>GSPSRKFYWRAKSQMCEVKGWVPTHRGFPWGPELPGDLILSRRAYVSCDLTSCFKFFIAYGLSANQHLLNTSMEWEESLYKTPIGSASTLSTSEMILPGRSSSACFDGLKWTVLVANGRDRNSFIMIKYGEEVTDTFSASRGGPLRLPNSECICIEGSCFVIVSDGPNVNQSVHRIYELQNGTVQRWKQLNTTGINFEYSTCYTINNLIKCTGTNLWNDAKRPLLRFTKELNYQIVEPCNGAPTDFPRGGLTTPSCKMAQEKGEGGIQGFILDEKPAWTSKTKAESSQNGFVLEQIPNGIESEGTVSLSYELFSNKRTGRSGFFQPKGDLISGCQRICF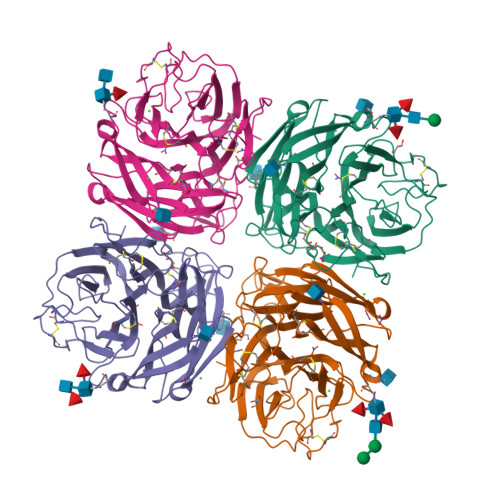WLEIEDQTVGLGMIQELSTFCGINSPVQNINWDS[6x]>QVLEGLDAVRKRPGMYIGSTDGAGLHHLVWEIVDNAVDEALSGFGDRIDVTINKDGSLTVQDHGRGMPTGMHAMGIPTVEVIFTILHAGGKFGQGGYKTSGGLHGVGSSVVNALSSWLEVEITRDGAVYKQRFENGGKPVTTLKKIG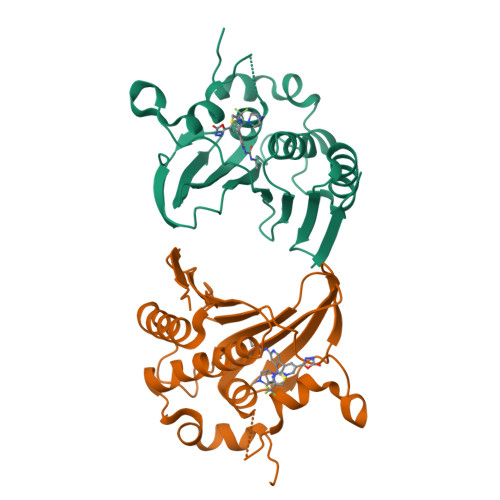TALKSKTGTKVTFMPDATIFSTTDFKYNTISERLNESAFLLKNVTLSLTDKRTDEAIEFHYEN[2x]[FeFe]-hydrogenases represent one of natures’ most effective classes of redox enzymes catalyzing the reversible reduction of protons to dihydrogen (H2) at turnover frequencies of up to 9000 s-11–3. With their low catalytic over-potential, [FeFe]-hydrogenases represent excellent models for a regenerative and likewise economically feasible H2 production. Their active center (“H-cluster”) can be structured into a standard [4Fe-4S]-cluster ([4Fe]H) and a diiron site ([2Fe]H). Theoretical studies suggest that the most probable PT pathway comprises of strictly conserved residues E282, S319, E279, and C299 (from surface to H-cluster, numbering corresponds to CpI), including two protein-bound water molecules (Wat826, Wat1120 4XDC19, chain B) located between E279 and C29915,16,20. In this study, site-directed mutagenesis (SDM) is used to investigate the PT pathway of two [FeFe]-hydrogenases, namely CpI and HydA1, which represent the largest (M3) and smallest (M1) type of monomeric [FeFe]-hydrogenases, respectively.

The strongest impacts were achieved when replacing E279CpI for A or Q, or C299CpI for A or S, resulting in activities <1%. Interestingly, the crystal structure of C299ACpI reveals that the removal of the thiol group causes an additional H2O molecule to occupy the vacant space. While the additional H2O is expected to rescue PT activity, it obviously does not restore enzymatic activity. Thus, an alternative proton acceptor has to be assumed. The additional H2O molecule (Wat962), which is trapped in the space of the missing thiol group of variant C299A would be a plausible proton acceptor. As it is well-positioned to bridge the adt-ligand (distance 3.4–3.7 Å) and Wat826 (distance 3.6–3.7 Å), it seems surprising that we are unable to measure any significant catalytic activity. This could be due to an unfavorable pKa difference among the Zundel-ion-like complex, the uncharged adt-ligand and glutamic acid E279Cp48. We assume that the proton is trapped in a Zundel-ion-like configuration with a dangling H2O molecule Wat962 downstream of position A299 that prevents E279 from being re-protonated (C299A).

>[2x]MKTIIINGVQFNTDEDTTILKFARDNNIDISALCFLNNCNNDINKCEICTVEVEGTGLVTACDTLIEDGMIINTNSDAVNEKIKSRISQLLDIHEFKCGPCNRRENCEFLKLVIKYKARASKPFLPKDKTEYVDERSKSLTVDRTKCLLCGRCVNACGKNTETYAMKFLNKNGKTIIGAEDEKCFDDTNCLLCGQCIIACPVAALSEKSHMDRVKNALNAPEKHVIVAMAPSVRASIGELFNMGFGVDVTGKIYTALRQLGFDKIFDINFGADMTIMEEATELVQRIENNGPFPMFTSACPGWVRQAENYYPELLNNLSSAKSPQQIFGTASKTYYPSISGLDPKNVFTVTVMPCTSKKFEADRPQMEKDGLRDIDAVITTRELAKMIKDAKIPFAKLEDSEADPAMGEYSGAGAIFGATGGVMEAALRSAKDFAENAELEDIEYKQVRGLNGIKEAEVEINNNKYNVAVINGASNLFKFMKSGMINEKQYHFIEVMACHGGCVNGGGQPHVNPKDLEKVDIKKVRASVLYNQDEHLSKRKSHENTALVKMYQNYFGKPGEGRAHEILHFKYKKSAWSHPQFEK> GSHMTQFAFVFPGQGSQTVGMLADMAASYPIVEETFAEASAALGYDLWALTQQGPAEELNKTWQTQPALLTASVALYRVWQQQGGKAPAMMAGHCLGEYSALVCAGVIDFADAVRLVEMRGKFMQEAVPEGTGAMAAIIGLDDASIAKACEEAAEGQVVSPVNFNSPGQV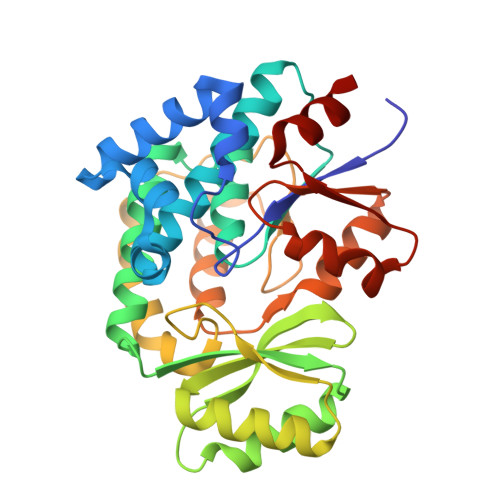VIAGHKEAVERAGAACKAAGAKRALPLPVSVPSHCALMKPAADKLAVELAKITFNAPTVPVVNNVDVKCETNGDAIRDALVRQLYNPVQWTKSVEYMAAQGVEHLYEVGPGKVLTGLTKRIVDTLTASALNEPSAMAAALEL> MLSSKYSKRIAWMKTTICDSLQLKDMIVEESFQYEKNKNLLEQFLSGEGLNKIFAYYQVQEQAQNDDIKDTGAQDPVLFFTTGDLEKIQDKAVWFLRITNPADDKKKASQQDGNDNDIIFGEITPNTVPMLNALMESVYSRQIDHIITEKIQFWGVAEEEQVLEFQQHSNKFSSEVREAINLMSPGTEHFKLDYEAISGLSESEKMQHYEMKFNEWINLISSQLNDDSEVRKDEKDAGPATELIYWRSRMQKITNWSEQLKSKDFQIVKASLQRHKNHDNQRPRGDESLSKLMMEYNRLDLLLTDKLNEAKDNVKYLTTLEKFIEPLYNGTPQQIIDTLPALMNAIKMIHTIARFYNTTDKMTGLFIKITNQMIKNCKDRILNKKDNGDNPSLYKMIWEQDPAELIEVLGSCIKLYCEYKKCYNDTKEKVADMPKGKTFDFSDAQIFGKFDTFVRRLQKLIEIFSNIQQFNALAKHNLEGMDVLTNKFKKIIDDFKKKGHNLLDTANNKFDRDWVEFNVEISHLDGELQNFIDNNFNRFRNIEYSLKLLHKFQSTIKRDSLKHNLTSRYNAILHNYATELDTIQRVFQDQKSNPPLVRNMPPEAGKIIWARHLFQKITGPINIFPENVINSTEIRRYYGSYNTLGKQLTIYEMWFYQDWVNKIEQSKAALQATLIVRHDENKKLYVNFDLEIMQLIREAKCLDRQGIEIPESARIILLQEDKFKTYYNELLYALKEYERINSKIKPICKNLLLPHIEDLDLKLRPGMVTLTWTSMNIESYLYYVHQGLKKLEQLIINVNDIIENRIENNLKTVSKVVLVHLPQDTKPLSLDSFVQLQEEYINSKTDFLTSKNVEVERAVDDLLQTIMLYPLDPHVDPVLPEETKRIKRYYFWYFYQALLNSTQNSLNAMKYRVCGKKIPGANTLQNLKPFFQVEVQLNGDKVTLNPSLQEIQKSINRAATAVLRCSKHLYNWDQQNKDSTDKATFYDMIACDKEIVKVILLLTGSIQGTKNKVNEFLSGFTKFEWLCKESIQESIKKFSKNGPTLQNYEDQLKKFSQIEEEIEKIVPTYKIGAMELMTHNICTSLSTWAKEWKLQYSQDLHKRARQLLDSLTEQTKMLSTKLSKPVKDIDSLGYVMETLEQIRKEQAEIDMKFNPVQEMYSLLDNYLPGGITDKDEMDARSLLRRNWDILIQQAEIKGKEYQHKQAIYLKELKQSIKDFTNQVSIFRRDYEKNGPMVEGISPAEAMERLRRFEDEYDVKYQMYKINARGENLFGLQNQKYPELEKTDAEIKNLNKLYNLYDSVIKNIQQFKEKSWQDVSKDDLAKMEEDAGKYGEQCSRLPKDLKEWQAYRDLKNYIDSLREQLPLIISLKKPSIMPRHWEKIKEITNTKLNYENPDQFYIEEIMGAKLLDFREDIEDITESADKQLKIRTGLDEINLYWNDMQFQFGIWGKRDVPCMLNGLIVGTILERLEEDQLQLSTFNSQRHVTPFKAEVENLIRTFSDVNDTLDMWVKVQKLWTSLEPVFTGGDIARQMPLQAKQFQGIDKNWMKIMEKAVETKKVIPCCQNDMLKDFLPDLNRKLEDCQKMLEAYLEGKRKKFPRFYFVSNPTLLKILSQGSEPTSIQEDFEKLFDAITKVTFESAKDKKNPALKQITQIQQVIGRNEENISLTGYYVKCEGNIEDWLKKLEQNMQQTLKDIASAAAQQVFQVGLKEFVSSQASQIALLGLQILWTSKVNEGLERLSRNERNAMDIKRNEIKEHMNILSSMCLEDLNGAVERTKVETLVTIQVHQKDISMDLKCKDVNDFEWQKQTRIAWKTDIDECIISITDWDSPYSYEFLGAKERLCITPLTDRCYITLAQAMSMYYGGAPAGPAGTGKTETVKDLGRTLGVFVVVTNCSDQHRYRDMAKIFKGLVQSGLWGCFDEFNRIDLEVLSVVAMQVESITTARKQHMKKFMFPEEEIEIELIPTVSYFITMNPGYAGRQELPENLKVLFRGVSMMVPDREIIIKVKLASVGYLQIDLLAKKFNVLYRLCEEQLSKQ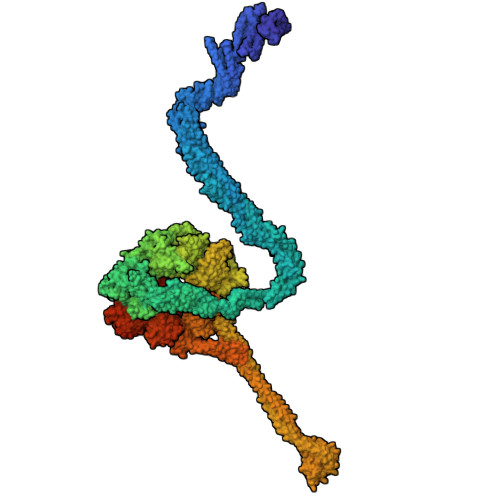RHYDFGLRNILSVLRTAGNTKRQEIKSDEEMLLMRSLRDMNLSKLVADDIPLFNGLLADIFPKLKEVPKKLYPDVEKKIPEEINAESYLINTPSFQLKIIQLYETCLVRHGFMLVGPTGSGKSTIMKILTEVLTKLGSPHKIVIMNPKAITAEQMYGVKSEISDDWIPGVFSTIWAKSNNRALKHTTWITCDGPVDAIWIENLNTVLDDNKILTLANGERIAMTENCKVVFEVENLNNASPATVSRCGQVYVSPTDLGYEAVIEGWIRNRKASGRAEESDKLGNILRKYLINMRFIELQSKECKEPMMDTSPVISVINILNLLTGCLQYFVQTQRTLSEQEYEKFIVYSMAWAIGGIYEAQDRVRFHELLLAKNAPIPQKGKENETVFDYYVSQDYLDWKICSPEEWVPPQSLQFSQLLLPTLDSFRAEMLLNFILTQPKSHTCSNSALLIGGSGTAKTSSVLLYCNKFDPQKMLFKRTNFSSATSPFMFQSTIEAECDFKVGKEFAPPGNKMMTIFIDDMSMPFVNKWGDQITLELVRQLIETGGFYMLDKTQRGNQRKMKNLQYIGAMNHPGGGRNDIPNRLKRQFFIFNMILPLSIEGIYGPIIKHMFKQKYFSDSTYKVIESLTSATIALWNKVKSTMLPTPAKFHYVFNMRELSRIFKGILTCKKDTINDAPKSMKIKPELFLVGLWRHEAERVLADKLVNNKDKDTVMGYIQEVSLESFSQIENEILEKYSSEKTFLFCDFLRPDVINEDGIIEEEAPKIYEAIDSLTELRKRCNFLLSFYNDRNPSKKMPLVLFDDALKHLLRISRIIRQPRSSGLLVGVGGSGKQSLTRLAGFIGKNLIQQIIVTKTYSDKDLKEDIKKGFDDAGHLGKQVTFLMTDSEVKKEEFLEYINMVLSTGEIPNLLAKDEREVWLGDISQAYCKEKNLGNIDPPQSELWTYFVDRVRDNFHIMLCFSPVGQKFRERARKFPALFNECTIDWFLPWPEEALVSVAETFIKNFDKLDTKEETKQELMKHMGNVHLMVNEICDEYYQKMRRQVYVTPKSFLSYLNSYKTLYIEKYDELDQQEESFKIGLNKIQEATITINQMEISLKEEEIQLNEATEKTNQLLANLDKESKKANQKGEEVAATNKQCEIQAEQISKEKEEAERELEAALPALRRAQEAVDSIESKDIVELKANKKPLDIIKYIMDAVLVFFKARLIPIQIEERVFNKKEGKAVLFLKESYDESGIQTLGDMNFMKKLKEFEKDSINEETIELLEPYLNQSEDWFNDTFATKASKAAAGILKWAFAIYEYHQKSKIVKPKRIQVAIAEGRQAIALKELEKAREDLAQIQAYIKNLKDVYTKQMEEKNELEMKAAKTKKKINTARTLITSLSGEKDRWGKGAQDISDQKRKLVGNVSLSTAFISYCGPFNAEYRNKLAQQRFVVDMKKRGVPVTPGLELTSFLIDDATIGEWNLQGLPKDDLSIQNGIMVTNSARYPLFIDPQGQGQNWIRNKLSASIIPERCITTLSHPKFKDMFLKYCMESGLTLIVENIENEVDPMMDPVLERQIIVKGKTQFVNVAGTEMELSKEFKLFMTCRLANPSFSPELSAKTTIIDFTVTQSGLEQQLLGKVISKEQKALEDSLNQLLADVNQNQKDLQRLDKNLLERLINSQGNLLDDTELMDVLNNTKTQAKEVAAKLIDAEIKTKEINEKREQYRPVAIRGSAIYFTMIEVSLVNWMYNSSLEQFLKLFIESIDLSEKAQLPSNRVKNIISFLTFHVYRYVNRGLFEKDKITFILMMAFKILTTAGTISSGDVSLFLKSGDALDIKSERQKQISYLEDNQWLNILALSKHTFSGQTLPFFKELPDLISRSENQWRNWIDKNDPENFPIPDFAESINQEKEIGSFISLCLVRSLRNDRTLIATQNFISNVLGKEFTDPISYPIEGIWQESSNMDPVLFLLSAGADPTSSIDELAKKKKKFPCEKVSMGEGQERVARQVIMKGFVEGGWVILQNCHLGLKFMEEIETLVSPINQIHEDFRLWITCEQHPKFPLGLLQKTLKVTNEPPKGLKAGLYKTFTTIITQEFIDKVDHSNWRSLIFTICFLHSIVIERKKFGPLGWCVPYEYNYSDLEASLLYIEKYLTNLMSTPQPNSHNLPISMNVVRYMICEVQYGGRITDDLDRELFITYGETYLKDGIFGNDYFFYDIMVDGSGQKFKYRIPQNPSAELIKYQEYIAKVPTVDNPEVFGLHSNADLTFRLKESKEMINTVMETRPKDSSVGGGKTREEIVQDKAKDMLKNLPPDYNDVEVRELVSKLGGPNPKTSTERGMTVPLNIFLYQEVTRMQRVIGLVRKTLQDTILAIDGQIIMTPEILEAINAIYDAKVPNSWLYDPSGAEISWLLPNLGSWSTSLSDRNKQLNDWLRSGQRPILFWLTGFFNPQGFLTGMKQEVTRNHKKKDGKGGEAWSLDDVVYSTTVKEREKEKDIEQPPAEGVYIKGLYLEGCKWSKNGLDDSDPKKIFADLPILHVSAINKKKTNEQDRMSNTYLCPVYKYPKRTDKYLIFRVGLPCEGSNNPSHWKLRGVALLCSTE> RSFSSRTPVNENPD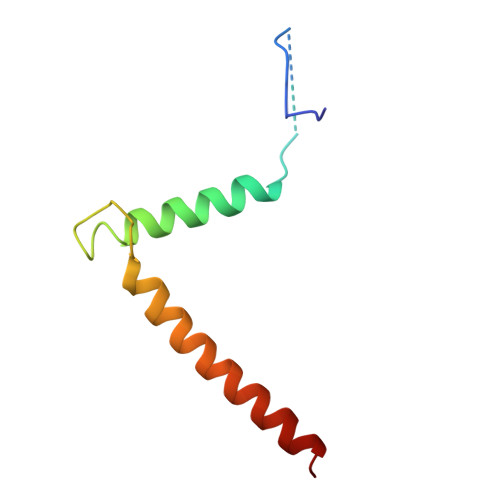GVQYRRGFVTRHQVSGWRFVMRRIASGVALHDTRMLVDPLRTQSRAVLTGALILVTGLVGCFIFS TEBIPENEM | C16 H21 N3 O4 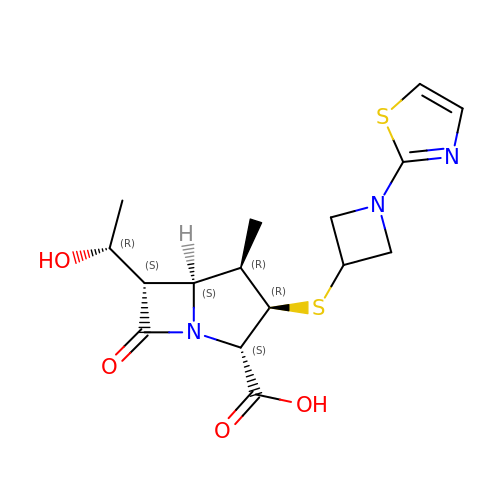S2 | YKLAKHLDAXNBOF-IOJHDDLYSA-N> SPVAPACDPRLLNKLLRDSHLLHSRLSQCPDVDPLSIPVLLPAVDFSLGEWKTQTEQSKAQDILGAVSLLLEGVMAARGQLEPSCLSSLLGQLSGQVRLLLGALQGLLGTQLPLQGRTTAHKDPNALFLSLQQLLRGKVRFLLLVEGPTLCVRRTLPTTAVPSENLYFQG;>QDVFLLALGTEPLNCFSQTFEDLTCFWDEEEAAPSGT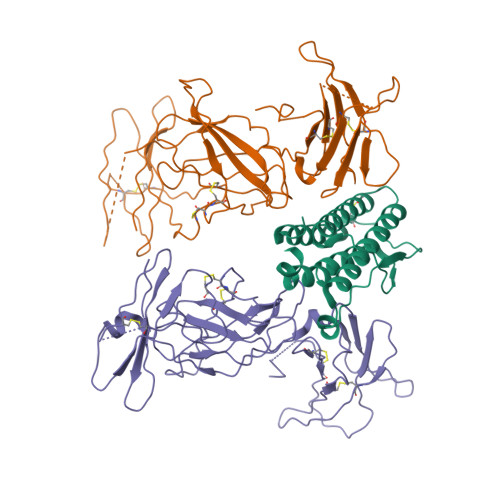YQLLYAYRGEKPRACPLYSQSVPTFGTRYVCQFPAQDEVRLFFPLHLWVKNVSLNQTLIQRVLFVDSVGLPAPPRVIKARGGSQPGELQIHWEAPAPEISDFLRHELRYGPTDSSNATAPSVIQLLSTETCCPTLWMPNPVPVLDQPPCVHPTASQPHGPAPFLTVKGGSCLVSGLQAGKSYWLQLRSQPDGVSLRGSWGPWSFPVTVDLPGDAVTIGLQCFTLDLKMVTCQWQQQDRTSSQGFFRHSRTRCCPTDRDPTWEKCEEEEPRPGSQPALVSRCHFKSRNDSVIHILVEVTTAQGAVHSYLGSPFWIHQAVLLPTPSLHWREVSSGRLELEWQHQSSWAAQETCYQLRYTGEGREDWKVLEPSLGARGGTLELRPRARYSLQLRARLNGPTYQGPWSAWSPPARVSTGSETAWENLYFQ[2x]> QIELEYKRKPIPDYDFM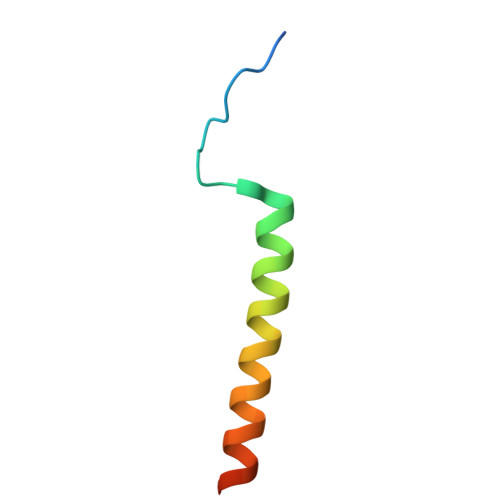KGLETTLQELYVEHQSKKRRLELFQLTN(2S)-3-[4-(acetylamino)phenoxy]-2-hydroxy-2-methyl-N-[4-nitro-3-(trifluoromethyl)phenyl]propanamide 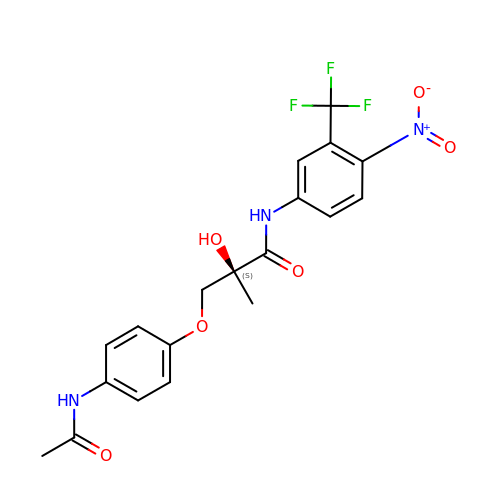| C19 H18 F3 N3 O6 | YVXVTLGIDOACBJ-SFHVURJKSA-N>MRGSHHHHHHGSACELGTDKAFITVLEMTPVLGTEIINYRDGMGRVLAQDVYAKDNLPPFPASVKDGYAVRAADGPGDRFIIGESQAGEQPTQTVMPGQVMRVTTGAPIPCGADAVVQVEDTELIRESDDGTEELEVRILVQARPGQDIRPIGHDIKRGECVLAKGTHMGPSEIGLLATVGVTEVEVNKFPVVAVMSTGNELLNPEDDLLPGKIRDSNRSTLLATIQEHGYPTINLGIVGDNPDDLLNALNEGISRADVIITSGGVSMGEKDYLKQVLDIDLHAQIHFGRVFMKPGLPTTFATLDIDGVRKIIFALPGNPVSAVVTCNLFVVPALRKMQGILDPRPTIIKARLSCDVKLDP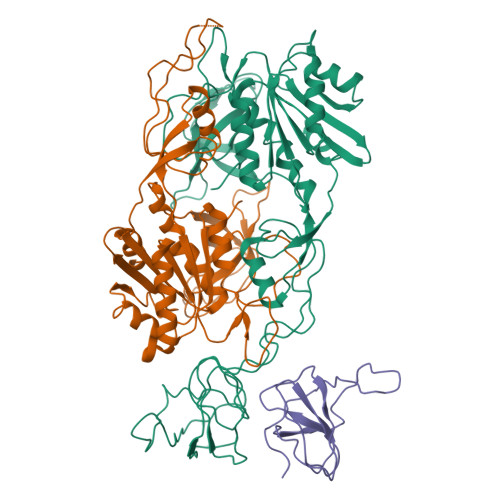RPEYHRCILTWHHQEPLPWAQSTGNQMSSRLMSMRSANGLLMLPPKTEQYVELHKGEVVDVMVIGRL[3x]Strong evidence has implicated the lipid kinase PI4KIIIβ, a phosphatidylinositol kinase widely expressed in mammalian cells, in the replication of several RNA viruses, including HRV, due to its signalling pathway. As a result, PI4KIIIβ is an appealing target for prevention of HRV-driven exacerbations in respiratory diseases. Inspired by the renaissance of covalent inhibition as a mechanism to target proteins of interest, this strategy was chosen for the development of inhibitors of PI4KIIIβ with a prolonged duration of action. The aim of this project was to develop a selective irreversible covalent inhibitor of PI4KIIIβ which targeted the conserved lysine (Lys549) in the ATP binding site.

Pleasingly, compound 4 covalently modified recombinant PI4KIIIβ protein. The incubation of an excess of 4 with the enzyme revealed only one covalent modification, indicative of a selective target engagement. The mass shift after covalent labelling was consistent with addition of 4 minus the fluoride ion, correlating with attack of a nucleophilic residue onto the electrophilic sulfur atom and expelling a fluoride leaving group. To gain further evidence that compound 4 covalently labelled Lys549, protein X-ray crystallography was used to characterise the adduct. Electron density consistent with 4 forming a covalent bond with Lys549 was observed. The oxygen linker of the fluorosulfate group directed the warhead to interact with Lys549; it is possible that rotation about the fluorosulfate warhead was restricted due to a steric clash with the o-methoxy substituent. Compound 4 bound through a hinge binding interaction between the valine backbone amide and the nitrogen donor/acceptor atoms of the heterocyclic core. In addition, the p-pyridyl head group formed a favourable hydrogen bonding interaction with Tyr385. The measured KI was 29.8 nM which means the reversible interactions were favourable and a low concentration of 4 was required to achieve 50% inhibition. Despite this, the irreversible step, forming a covalent bond (described by kinact), was measured to be 1.17 × 10−4 s−1, which is orders of magnitude slower than literature precedent for a lipid kinase, thus, the rate of covalent bond formation was deemed to be slow.

> GRTASNPKVENEDEPVRLAPEREFIKSLMAIGKRLATLPTKEQKTQRLISELSLLNHKLPARVWLPTAGFDHHVVRVPHTQAVVLNSKDKAPYLIYVEVLECENFDTTSVPARIPENRIQSTQSVETAFKRDPEDPSAVALKEPWQEKVRRIREGSPYGHLPNWRLLSVIVKCGDDLRQELLAFQVLKQLQSIWEQERVPLWIKPYKILVISADSGMIEPVVNAVSIHQVKKQSQLSLLDYFLQEHGSYTTEAFLSAQRNFVQSCAGYCLVCYLLQVKDRHNGNILLDAEGHIIHIDFGFILSSSPRNLGFETSAFKLTTEFVDVMGGLDGDMFNYYKMLMLQGLIAARKHMDKVVQIVEIMQQGSQLPCFHGSSTIRNLKERFHMSMTEEQLQLLVEQMVDGSMRSITTKLYDGFQYLTNGIM>MGPPEKDSKAILKARGLEEEQKSESTMSPSENVSRAILKDSGSEEVEQASERKMTSPENDSKSIQKDQGPEQEQTSETLQSKEEDEVTEADKDNGGDLQDYKAHVIAKFDTSVDLHYDSPEMKLLSDAFKPYQKTFQPHTIILHGRPGVGKSALARSIVLGWAQGKLFQKMSFVIFFSVREIKWTEKSSLAQLIAKECPDSWDLVTKIMSQPERLLFVIDGLDDMDSVLQHDDMTLSRDWKDEQPIYILMYSLLRKALLPQSFLIITTRNTGLEKLKSMVVSPLYILVEGLSASRRSQLVLENISNESDRIQVFHSLIENHQLFDQCQAPSVCSLVCEALQLQKKLGKRCTLPCQTLTGLYATLVFHQLTLKRPSQSALSQEEQITLVGLCMMAAEGVWTMRSVFYDDDLKNYSLKESEILALFHMNILLQVGHNSEQCYVFSHLSLQDFFAALYYVLEGLEEWNQHFCFIENQRSIMEVKRTDDTRLLGMKRFLFGLMNKDILKTLEVLFEYPVIPTVEQKLQHWVSLIAQQVNGTSPMDTLDAFYCLFESQDEEFVGGALKRFQEVWLLINQKMDLKVSSYCLKHCQNLKAIRVDIRDLLSVDNTLELCPVVTVQETQCKPLLMEWWGNFCSVLGSLRNLKELDLGDSILSQRAMKILCLELRNQSCRIQKLTFKSAEVVSGLKHLWKLLFSNQNLKYLNLGNTPMKDDDMKLACEALKHPKCSVETLRLDSCELTIIGYEMISTLLISTTRLKCLSLAKNRVGVKSMISLGNALSSSMCLLQKLILDNCGLTPASCHLLVSALFSNQNLTHLCLSNNSLGTEGVQQLCQFLRNPECALQRLILNHCNIVDDAYGFLAMRLANNTKLTHLSLTMNPVGDGAMKLLCEALKEPTCYLQELELVDCQLTQNCCEDLAC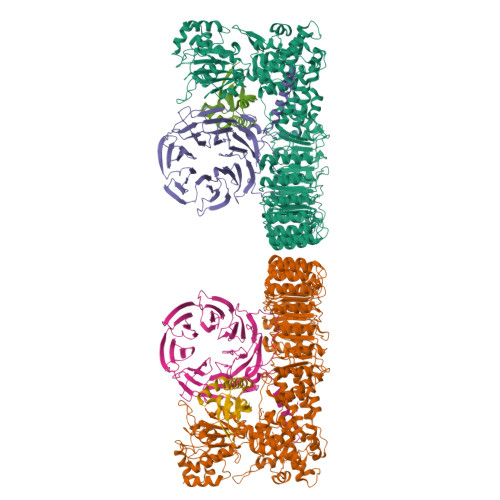MITTTKHLKSLDLGNNALGDKGVITLCEGLKQSSSSLRRLGLGACKLTSNCCEALSLAISCNPHLNSLNLVKNDFSTSGMLKLCSAFQCPVSNLGIIGLWKQEYYARVRRQLEEVEFVKPHVVIDGDWYASDEDDRNWWKN[2x];>[2x]MTSHRQSSDTFGGILPSTLSSRYLSIVNQLPEEFSSVVSEMMVHLENIFSLAENFFQAIERFSRTPDLLERNKMSIGVGAEGDSWPCHVSHEAPMGSAQTTENSAKEEDKQVPESAALQHPKFKSTPGPQLPTRRRFLSESDELQDPQPVWDAEPQFCQGFLIQGLWELFMDSRQKNQQEHGGEDSSQESKDSGLCDFKPEPQPRHRNSLSDSADPFLIKSPSALLDYYQEDVSRPQPETQESSGRADKFLKPLSWGSEVLESSCNQPSTALWQLERFTVPQALQKVRVLKHQELLLVVAVSSFTRHVFTCSQSGIKVWNLVNQVAEDRDPESHLKCSVQDNKVYLRTCLLSSNSRTLFAGGYNLPGVIVWDLAAPSLYEKCQLPCEGLSCQALANTKENMALAGFTDGTVRIWDLRTQEIVRNLKGPTNSARNLVVKDDNIWTGGLDACLRCWDLRMAKVSLEHLFQSQIMSLAHSPTEDWLLLGLANGQHCLFNSRKRDQVLTVDTKDNTILGLKFSPNGKWWASVGMGNFITVHSMPTGAKLFQVPEVGPVRCFDMTENGRLIITGSRDCASVYHIKY;>MASHTADADAKPDSDSQKLLNVLPVSLRLRTRPWWFPIQEVSNPLVLYMEAWVAERVIGTDQAEISEIEWMCQALLTVDSVNSGNLAEITIFGQPSAQTRMKNILLNMAAWHKENELQRAVKVKEVEEFLKIRASSILSKLSKKGLKLAGFPLPLEGRETQMES[2x]> DLFTLSFSPDLSIASEAEQLTLQSKDDRLILEHPQPGLRTALEQLKQGNLTLAQLTELVSEQDGVEAGITFASELEKLVDLGWICHSVLPLITAIPIAKDYELNVPDSSWQTTAIALSRFA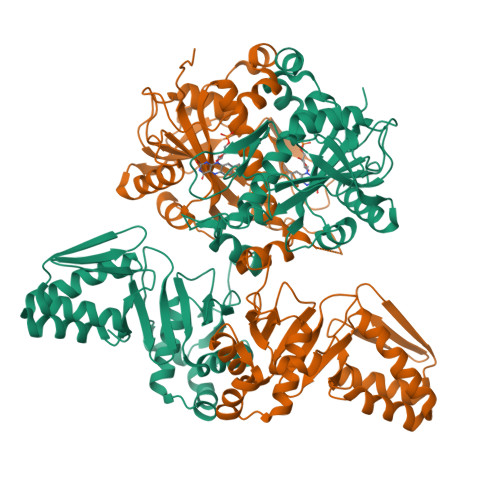FLHQDLQQLVLESPRSKSKLVILDWRVGAVIAKLAQSDRGFIFATSADSLLADLSLELEELKRLFALLIATQMMDLEPEDETITQWKFHNLLFHHYTRLGRLDNSRKLNLPVFEHRDRYPYVKPVISTQAIPLVKPDLTALATTDMTLTEAIETRRSIREYSDQPITLAQLGEFLYRCARVKAVYTLPEDPMQVGESTTRPYPSGGALYELEIYPLVHQCGDLAAGLYHYQPLSHTLHPVADWTPEVESLVYDAWRATGQQSIPQIVLIITARFGRLFWKYHDIAYSLILKHVGVLYQTFYLVATAMQLAPSAIGAGNTTKFCQIAGLNPDEEASVGEFSLGAAKP;> MLDLFTLSFSPDLSIASEAEQLTLQSKDDRLILEHPQPGLRTALEQLKQGNLTLAQLTELVSEQDGVEAGITFASELEKLVDLGWICHSVLPLITAIPIAKDYELNVPDSSWQTTAIALSRFAFLHQDLQQLVLESPRSKSKLVILDWRVGAVIAKLAQSDRGFIFATSADSLLADLSLELEELKRLFALLIATQMMDLEPEDETITQWKFHNLLFHHYTRLGRLDNSRKLNLPVFEHRDRYPYVKPVISTQAIPLVKPDLTALATTDMTLTEAIETRRSIREYSDQPITLAQLGEFLYRCARVKAVYTLPEDPMQVGESTTRPYPSGGALYELEIYPLVHQCGDLAAGLYHYQPLSHTLHPVADWTPEVESLVYDAWRATGQQSIPQIVLIITARFGRLFWKYHDIAYSLILKHVGVLYQTFYLVATAMQLAPSAIGAGNTTKFCQIAGLNPDEEASVGEFSLGAAKPQQQS>SMKTILVTAFDPFGGEAINPSWEAIKPLQGSQVFGANIEICQIPCIFDTSLEHLYAAVDKYQPELVISVGQAGGRTNITVERVAININDARIPDNAGNQPIDTPVIVDGPAAYFSRLPIKTMVNALNTAGIPASVSQTAGTFVCNHVMYGLLHYLAQNTPSVRGGFIHVPYLPEQAVKDGNQSSMTLMLMTL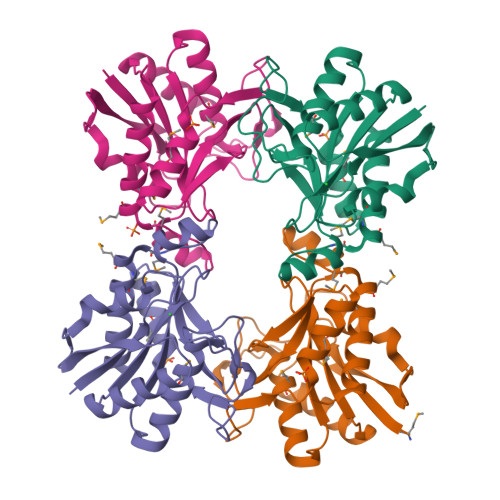ALKIAIETAWKNTSDIAVTGGATH[4x]> MAHHHHHHAFWIQGPGNAFYQKQGESRYQRTLELPATRGKILDRNGLVLATSLPVRAIWAIPDAVPDDLGADKINQLGKLLGMTPKELRVKLSEDKGFVYVKRQVPIDVADKVAALDIPGIYQRNEYKRFYPEGEITAHLIGFTNVEDEGQEGVELGDQKLLSGTSGVRRVIKDRLGHIVEDVAEQVPPHNGTDVGLSIDSKIQYIAYANLKAAVEKFKAKAGAAMVVDVRTGEVLALVNYPTYNPNDRTRLTGEQLRNRILTDVFEPGSIMKPFTVSLALDLHRVTPNTLVETGNGHFVLDGAPITDDAGFGTLTVGGVIQKSSNIGATKIAMTMRPEEM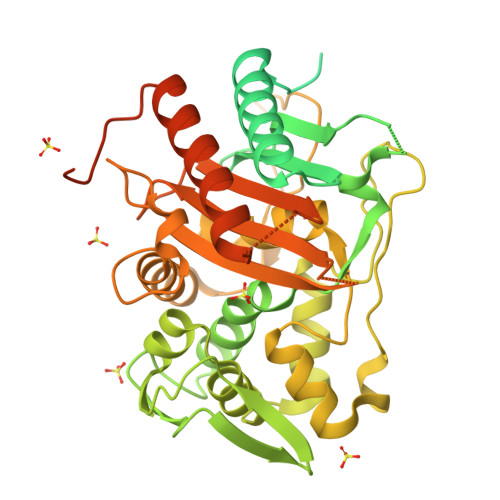WNMYTSIGLGQAPKVGFPGAAAGRLRPWKSWRRIEQATMSYGYGLSVSLFQLARAYTAIAHDGEMMPVTIFKTDPNQQITGTQVFTPTTAREVRTMLETVVAPGGTSPDAAVPGYRVGGKSGTAYKHEGHGYTRKYRASFVGMAPMPNPRIVVAVSVDEPTAGSHFGGQVSGPVFSAIAGDTMRALNVPPNMPIKQLVVSDDAPGAPAKPGPQKLAAGSGAKHMIVSSTTRNSPGVVR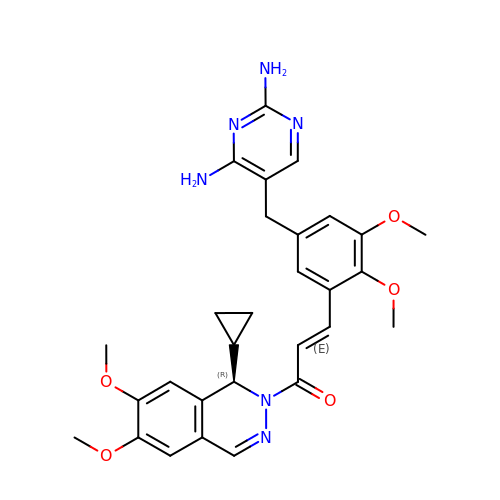(2E)-1-[(1R)-1-cyclopropyl-6,7-dimethoxyphthalazin-2(1H)-yl]-3-{5-[(2,4-diaminopyrimidin-5-yl)methyl]-2,3-dimethoxyphenyl}prop-2-en-1-one | C29 H32 N6 O5 | WEOHMFQXNAIIAE-DIJOXEGBSA-N>[2x]TATYSGNPFVGVTPWANAYYASEVSSLAIPSLTGAMATAAAAVAKVPSFMWLDTLDKTPLMEQTLADIRTANKNGGN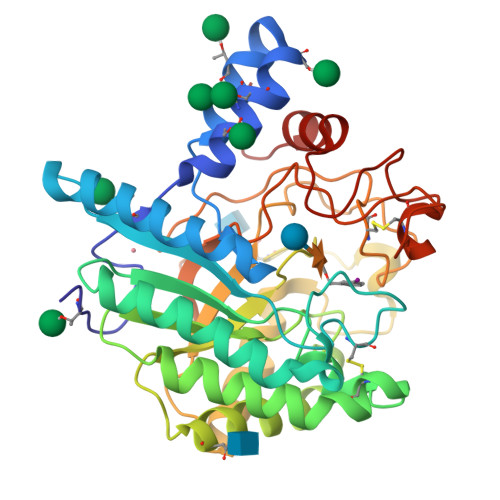YAGQFVVYDLPDRDCAALASNGEYSIADGGVAKYKNYIDTIRQIVVEYSDIRTLLVIEPDSLANLVTNLGTPKCANAQSAYLECINYAVTQLNLPNVAMYLDAGHAGWLGWPANQDPAAQLFANVYKNASSPRALRGLATNVANYNGWNITSPPSYTQGNAVYNEKLYIHAIGPLLANHGWSNAFFITDQGRSGKQPTGQQQWGDWCNVIGTGFGIRPSANTGDSLLDSFVWVKPGGECDGTSDSSAPRFDSHCALPDALQPAPQAGAWFQAYFVQLLTNANPSFL>AENYHLKWDSHLTYLNSSIATLYKNEKFADVVLYSSYNSSGIPSDIPTVGISAHKFILSASSQFFATMFETAPITNPNGVLYVVLPPDLSHRAIQI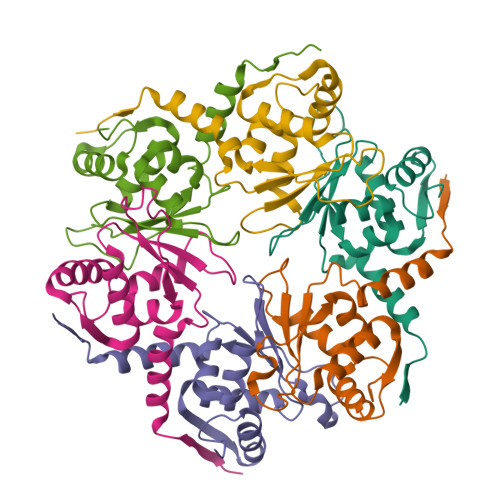LVQYMYSGEATVSNDILNEVLRGGEILKIRGLCRT[6x]>GNSPASVLGITANTWKINSFIGSPGSSATYYDDITDASGISYNTYSDDNYFYTDGEWVYFKCYRGLGGSANSQNPRVELREMDNGNLASWTGDSGTHTMEWTVQVNQLPQDTDGDGGVLCFGQIHGPSKNSD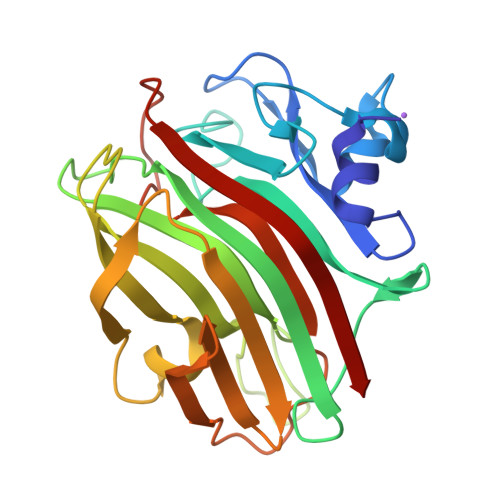GVEVDDVVRVQFIGEENQSSGSVKLKISGYVTEEQGGSQTFSGYSLDTTYNCKLVYSGGYVELFMNGSSVFRKKMEVDDLSENYFKVGNYLQSVKGASYTGSYGLVRIKNLSVTHN[2x]> MGSSHHHHHHSSGENLYFQGGTMYDFEYLNGLSYTELTNLIKNIKWNQINGLFNYSTGSQKFFGDKNRVQAIINALQESGRTYTANDMKGIETFTEVLRAGFYLGYYNDGLSYLNDRNFQDKCIPAMIAIQKNPNFKLGTAVQDEVITSLGKLIGNASANAEVVNNCVPVLKQFRENLNQYAPDYVKGTAVNELIKGIEFDFSGAAYEKDVKTMPWYGKIDPFINELKALGLYGNITSATEWASD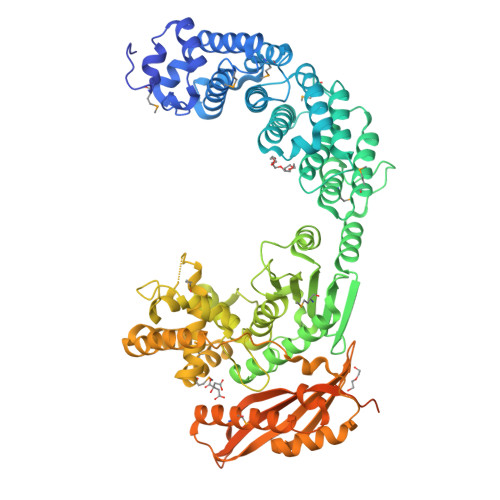VGIYYLSKFGLYSTNRNDIVQSLEKAVDMYKYGKIAFVAMERITWDYDGIGSNGKKVDHDKFLDDAEKHYLPKTYTFDNGTFIIRAGDKVSEEKIKRLYWASREVKSQFHRVVGNDKALEVGNADDVLTMKIFNSPEEYKFNTNINGVSTDNGGLYIEPRGTFYTYERTPQQSIFSLEELFRHEYTHYLQARYLVDGLWGQGPFYEKNRLTWFDEGTAEFFAGSTRTSGVLPRKLILGYLAKDKVDHRYSLKKTLNSGYDDSDWMFYNYGFAVAHYLYEKDMPTFIKMNKAILNTDVKSYDEIIKKLSDDANKNTEYQNHIQELVDKYQGAGIPLVSDDYLKDHGYKKASEVYSEISKAASLTNTSVTAEKSQYFNTFTLRGTYTGETSKGEFKDWDEMSKKLDGTLESLAKNSWSGYKTLTAYFTNYRVTSDNKVQYDVVFHGVLTDNGDISNNKAPIAKVTGPSTGAVGRNIEFSGKDSKDEDGKIVSYDWDFGDGATSRGKNSVHAYKKAGTYNVTLKVTDDKGATATESFTIEIKN>[4x]S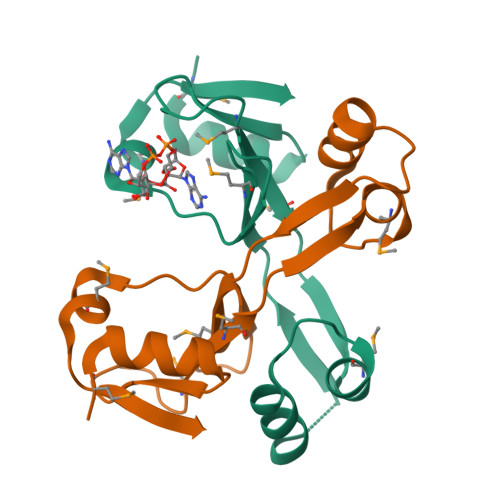MTFGQALESLKRGHLVARKGWNGKGMFIFMRPEDSLPTNMIVNQVKSLPESFKRWVANNHGDSETDRIKFTAYLCMKAADGTIVNGWLASQTDMLANDWVIVE>MHTLYAPGGYDIMGYLIQIMNRPNPQVELGPVDTSCALILCDLKQKDTPIVYASEAFLYMTGYSNAEVLGRNCRFLQSPDGMVKPKSTRKYVDSNTINTMRKAIDRNAEVQVEVVNFKKNGQRFVNFLTMIPVRDETGEYRYSMGFQC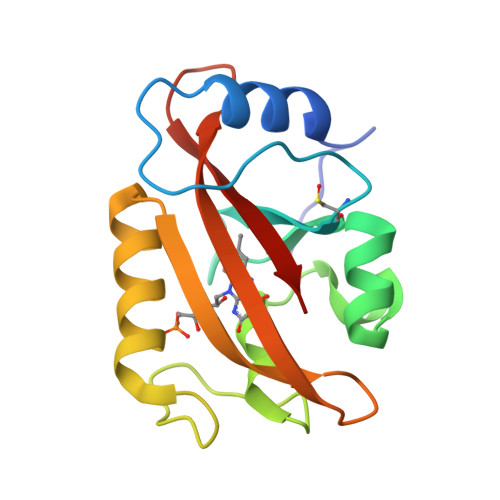ETE[4x]> AVY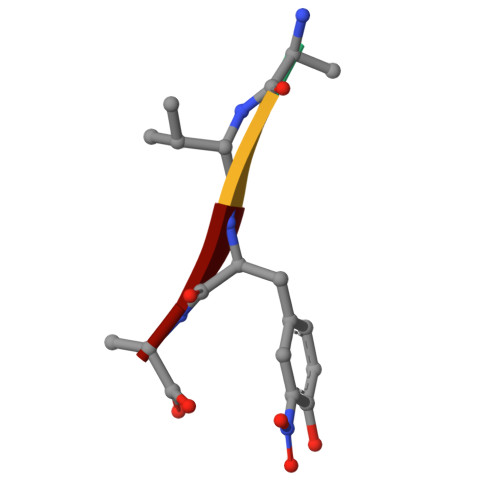A> MDKLLSSLENIEVDNILKTAREFKEDTCEEKINLSIGVCCNDDGDLHIFDSVLNADKLVTENYKEKPYLLGNGTEDFSTLTQNLIFGNNSKYIEDKKICTIQCIGGTGAIFVLLEFLKMLNVETLYVTNPPYINHVNMIESRGFNLKYINFFDYNLIDINYDLFLNDLRNIPNGSSVILQISCYNPCSVNIEEKYFDEIIEIVLHKKHVIIFDIAYQGFGHTNLEEDVLLIRKFEEKNIAFSVCQSFSKNMSLYGE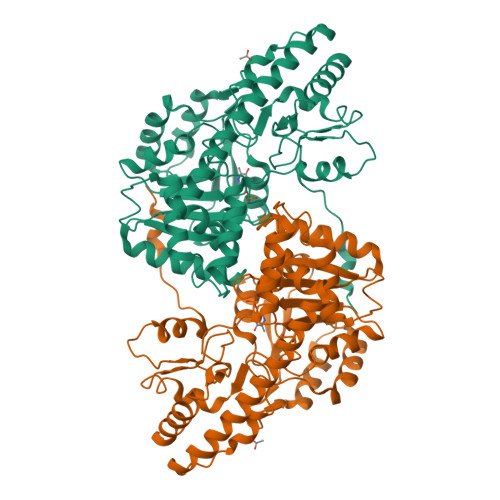RAGALHIVCKNQEEKKIVFNNLCFIVRKFYSSPVIHTNRILCQLLNNQNLKLNWIKELSQLSQRITNNRILFFNKLETYQKKYNLNYDWNVYKKQRGLFSFVPLLAKIAEHLKTHHIYIINNGRINVSGITKNNVDYIADKICLSLSQI>MEDINFASLAPRHGTRPFMGTWNEIGTSQLNGGAFNWSSVWSGLKNFGSTLRTYGNKAWNSSTGQLLREKLKDQNFQQKVVDGLASGINGVVDIANQAVQREINSRLDPRPPTVVEMEDATLPPPKGEKRPRPDAEETILQVDEPPSYEEAVKAGMPTTRIIAPLATGVMKPATLDLPPPPAPAPPKATPVVQAPPVATAVRRVPARRQAQNWQSTLHSIVGLGVKSLKRRRCY[8x];>[12x]MMPQWAYMHIAGQDASEYLSPGLVQFARATDTYFSLGNKFRNPTVAPTHDVTTDRSQRLTLRFVPVDREDTTYSYKARFTLAVGDNRVLDMASTYFDIRGVLDRGPSFKPYSGTAYNSLAPKSAPNPSQWTANEKQTGGQPKSVTQTFGSAPMGGSNITIEGLVIGTKEEEGNATEEIFADKTFQPEPQVGEENWQETEAFYGGRALKKDTKMKPCYGSFARPTNEKGGQAKLKLNDQGQPTKDYDIDLAFFDTPGGTPPTGSGQQEEYKADIVMYTENVNLETPDTHVVYKPGKEDESSETNLTQQSMPNRPNYIGFRDNFVGLMYYNSTGNMGVLAGQASQLNAVVDLQDRNTELSYQLLLDSLGDRTRYFSMWNSAVDSYDPDVRII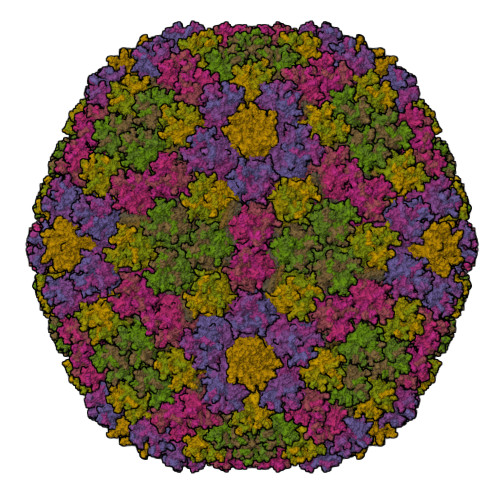ENHGVEDELPNYCFPLNGTGTNSTYQGVKVKTGQDGAEETEWDKDETVARQNQIAKGNVYAMEINLQANLWKSFLYSNVALYLPDSYKYTPANVTLPANTNTYEYMNGRVVAPSLVDAYINIGARWSLDPMDNVNPFNHHRNAGLRYRSMLLGNGRYVPFHIQVPQKFFAIKNLLLLPGSYTYEWNFRKDVNMILQSSLGNDLRVDGASVRFDSVNLYATFFPMAHNTASTLEAMLRNDTNDQSFNDYLSAANMLYPIPAKATNVPISIPSRNWAAFRGWSFTRLKTKETPSLGSGFDPYFVYSGSIPYLDGTFYLNHTFKKVSIMFDSSVSWPGNDRLLTPNEFEIKRSVDGEGYNVAQCNMTKDWFLVQMLSHYNIGYQGFHVPEGYKDRMYSFFRNFQPMSRQVVDEINYKDYKAVTLPFQHNNSGFTGYLAPTMRQGQPYPANFPYPLIGQTAVPSVTQKKFLCDRVMWRIPFSSNFMSMGALTDLGQNMLYANSAHALDMTFEVDPMDEPTLLYLLFEVFDVVRVHQPHRGVIEAVYLRTPFSAGN;> MRRAVVSSSPPPSYESVMAQATLEVPFVPPRYMAPTEGRNSIRYSELAPQYDTTRVYLVDNKSADIASLNYQNDHSNFLTTVVQNNDFTPAEASTQTINFDERSRWGGDLKTILHTNMPNVNEYMFTSKFKARVMVARKHPEGVVETDLSQDKLEYEWFEFTLPEGNFSETMTIDLMNNAILENYLQVGRQNGVLESDIGVKFDSRNFKLGWDPVTKLVMPGVYTYEAFHPDVVLLPGCGVDFTESRLSNLLGIRKKQPFQEGFRIMYEDLEGGNIPALLDVPKYLESKKKVEDETKNAAAATADTTTRGDTFATPAQETAADKKVEVLPIEKDESGRSYNLIQGTHDTLYRSWYLSYTYGDPEKGVQSWTLLTTPDVTCGAEQVYWSLPDLMQDPVTFRSTQQVSNYPVVGAELMPFRAKSFYNDLAVYSQLIRSYTSLTHVFNRFPDNQILCRPPAPTITTVSENVPALTDHGTLPLRSSIRGVQRVTVTDARRRTCPYVYKALGIVAPRVLSSRTF;> MQQAPDPAIRAALQSQPSGIASDDWEAAMQRIMALTTRNPESFRQQPQANRLSAILEAVVPSRTNPTHEKVLAIVNALAENKAIRPDEAGLVYNALLERVGRYNSTNVQSNLDRLVTDVREAVAQRERFKNEGLGSLVALNAFLATQPANVPRGQDDYTNFISALRLMVTEVPQSEVYQSGPDYFFQTSRQGLQTVNLSQAFKNLRGLWGVQAPVGDRSTVSSLLTPNSRLLLLLIAPFTDSGSVNRNSYLGHLLTLYREAIGQAQVDEQTFQEITSVSRALGQNDTDSLRATLNFLLTNRQQKIPAQYALSAEEERILRYVQQSVGLFLMQEGATPSAALDMTARNMEPSMYAANRPFINKLMDYLHRAAVMNTDYFTNAILNPHWLPPPGFYTGEYDMPDPNDGFLWDDVDSVVFSPTFQKRQEAPPSEGAVGRSPFPSLGSLHSLPGSVNSGRVSRPRLLGEDEYLNDSLLQPPRAKNAMANNGIESLVDKLNRWKTYAQDHRDAPAPRRQRHDRQRGLVWDDEDSADDSSVLDLGGSGGVNPFAHLQPKLGRRMF;>[2x]MSKEIPTPYMWSYQPQMGLAAGASQDYSTRMNWLSAGPSMISRVNGVRNHRNQILLEQAAVTSTPRAKLNPRNWPSTLVYQEIPGPTTVLLPRDALAEVRMTNSGVQLAGGASRCPLRPQSGIKTLVIRGRGTQLNDELVSSSIGLRPDGVFQLAGAGRSSFTPNQAYLTLQSSSSEPRSGGIGTLQFVEEFVPSVYFNPFSGSPGLYPDEFIPNFDAVREAVDGYD;>MNGTGGAFEGGLFSPYLTTRLPGWAGVRQNVMGSTVDGRPVLPANSSTMTYATVGSSSLDSTAAAAAAAAAMTATRLASSYMPSSGSSPSVPSSIIAEEKLLALLAELEALSRQLAALTQQVSELREQQQQQNK[4x]> MGPLQCHMQAFNANIISVDAYSANDLSDKHAPLGASGYFADVTLTGKYHQD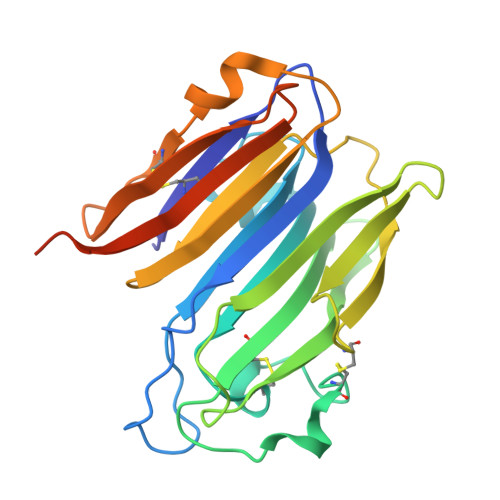VFDARHWLTMRHSGTDCRNVKGTDSKVCNIDYVENQPGNSCAQVTQRSHLLGWSSGKALDISATAPNAPVHFRASLAPSLQTWWTGLPNTCAVQRYNAPHNPYKIVTLTASGMHTWTKLVIMLDAPEPSFFKSWSCEYNDSLSPVVGNIQVSEDGKTYTLTNVKYQPILYSANEENKSLEHHHHHH REL-(3AR,4S,7R,7AS)-3A,4,7,7A-TETRAHYDRO-2-(4-NITRO-1-NAPHTHALENYL)-4,7-ETHANO-1H-ISOINDOLE-1,3(2H)-DIONE | C20 H18 N2 O4 | 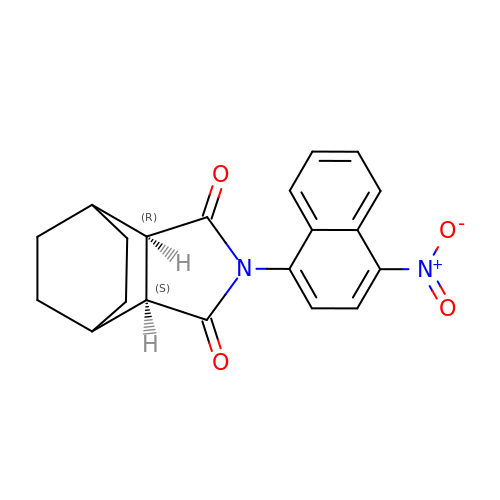DEJXHCDDTLTVNB-FRVJLOGJSA-N>[2x]MKQ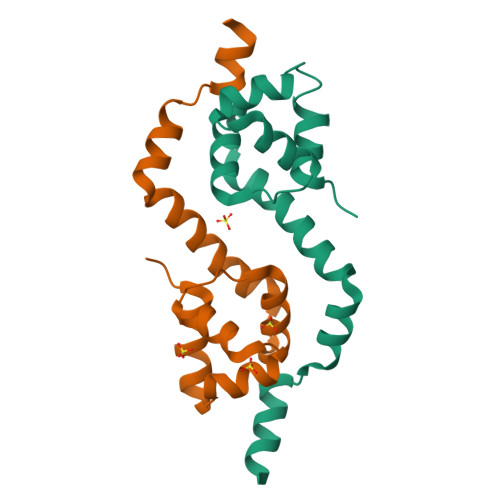ATRKPTTPGDILLYEYLEPLDLKINELAELLHVHRNSVSALINNNRKLTTEMAFRLAKVFDTTVDFWLNLQAAVDLWEVENNMRTQEELGRIETVAEYLARREERAKKVA The capsular polysaccharides (CPSs) surrounding the A. baumannii cells are the primary receptors for bacteriophages encoding specific structural depolymerases that determine the initial step of phage–host interaction. The genomes of Friunaviruses encode only one tailspike depolymerase (TSD) specific to a certain K type or several K types with similar structures or linkages between K units. In the obtained trimeric structures of the TSDs APK09_gp48, APK14_gp49, and APK16_gp47, each chain contains a particle-binding N-terminal domain and a central β-helix domain, as well as a C-terminal domain forming CPS-recognizing/degrading parts. All depolymerases studied were specific glycosidases that cleaved the corresponding CPSs by the hydrolytic mechanism with the production of monomers or/and oligomers (dimers and trimers) of the repeating K units.

APK14_gp49 structure consists of an N-terminal domain (residues 153–277) that possesses two α-helices (167–173 and 261–274) as well as four stranded β-sheet (176–241), a central β-helix domain (278–730) having 14 rungs and a C-terminal six-stranded β-barrel domain (731–851). Rungs 6–12 of the central β-helix domain are rungs, where B1, B3, and T3 are solvent-exposed, and T2 faces the three-fold symmetry axis of the trimer. Rungs 1–5 have only two β-strands, B2 and B3, and rungs 13–14 lack B2 and possess only B1 and B3. The APK14_gp49 β-helix domain is stabilized by 10 salt bridges, 79 hydrogen bonds, and hydrophobic interactions in a manner similar to those of APK16_gp47. APK14_gp49 crystallographic trimer has a diameter of 75Å and a length of about 150Å. Each subunit of the trimer has an interface area of about 2948Å2 (11% of the total subunit area). The trimer is dominantly stabilized by polar interactions, including a total of 105 hydrogen bonds and 15 salt bridges, while the hydrophobic impact is relatively small. The trimer has two non-interacting cavities in the central β-helix domain and one cavity in the N-terminal domain. In contrast to TSD APK16_gp47, in the APK14_gp49 trimer, the central cavities contain solvent molecules. Cleavage of the A. baumannii AB5256 CPS with depolymerase APK14_gp49 resulted in monomer 3 and dimer 4 of the K unit.

> GSDAAEEAAQVTRSADKVIDESGATQQELNNHSVQHVETVADLPTNAKDGAVLYVKGYYKPTNLALAKPYKGGSTRVYVAQRKDEDDGFLCIRGWVLQSETSIYTPHMSGCLCDGTTDDTLNFDKLMYALEKNNIAGKVIINDDMFFNSQCPRIGKLIDPVQFNEKNAIRLVSNVDLEINATLNFGPFFAGSSTQPRCNILSAMYREDVNDWYGKNRHENIKVYGTGTLDFTQTESPNAVQDGYRWIIKASVKGMEVYGLTFKGGDFANAIQTSKTSEHIRIYGNTFSNLMSDKSLLHDHSTIYCIGKDIKVHDNVFEFTNVKGRLNACACELHGSEQWFYKNVVRGYPNLVFSAILRTDQSLDENEVVYDQKAFDNTAFISRSALGYWSLANKSAKLRDLEFYDNTVTFIEAPTLAQYTSAGVRGLQYPSDLSASVFTTWLEGDTVPNVNYLAEVLDHILMKGNTFTASTGILQNQLVSIFRFVGCYVRENVKFIGNTVRVNTILNRDVSTGTTNDYFKGWVVTGNNYDFSMFRNQRHGLWIFLEYISGCVFDFNIKSRFPTLDKTYNLVNFVLRDKSKVVDNTINIDPNGSYAVLDSWLGGDFLTYTATDMGGRNNHIQSVAFVYINETRRKDSVFAKMGVQSGSIPPSVNMCSVIEYTNVMLGTVSYPVGFNKDYSAAYKLTATAIASQPFLDDETSDRFAYVHFKC Colicin E1 is a bacteriocin produced by, and lethal to, Escherichia coli that hijacks the outer membrane proteins (OMPs) TolC and BtuB to enter the cell. Colicin E1 is a bacteriocin produced by E. coli that enters the periplasm of neighboring cells and forms a pore on the cytoplasmic membrane leading to membrane depolarization and cell death. Unlike any of the other E colicins, the T domain of Colicin E1 binds to TolC, the outer membrane component of the acridine efflux pump, and the R domain binds BtuB, the primary receptor shared by all E colicins. TolC forms a large rigid conduit in the outer membrane and periplasm with a water-filled lumen.

We find that colicin E1 binds stably to TolC, not as a helical hairpin but as a single-pass folded helix with the N-terminus inside the periplasm. When resolved by cryoEM, addition of ColE1-T to TolC breaks the threefold channel symmetry and the additional protein is observed running all the way through the TolC barrel as a single-pass, all-α-helical chain spanning more than 130 Å. The ColE1 T domain inserts into TolC with its amino terminus pointing inwards through the periplasmic iris, and 2D class averages show that the carboxy terminus of the helix continues and projects out into the extracellular space. About 85 of the 190 ColE1-T residues could be modeled to this density (residues 46–131). The ColE1 chain binds TolC asymmetrically, primarily contacting only one of the three TolC chains. However, our cryoEM reconstruction of colicin E1 in complex with TolC shows that ColE1-T hinges open at the TolC box to an extended conformation upon binding to TolC (bottom). Compared to the unbound state, asymmetric ColE1 binding dilates the periplasmic TolC aperture and, makes only minor adjustments to the loops on the extracellular aperture so that they can accommodate ColE1 in the absence of any other proteins or motive force. The acidic patch of colicin E1 near the extracellular aperture contains two arginine residues (R129 and R131) that form hydrogen bond networks with one TolC chain each. In addition, colicin E1 residues T113, A116, N119, and N120 (all part of the TolC box) establish polar interactions with TolC residues G67, D69, S90, and K305 on one TolC chain (light red and light blue) while colicin H117 interacts with TolC F310 on a neighboring TolC chain (light red and light gold). By contrast with the β-barrel of TolC, in the interior of the periplasmic helical barrel of TolC, colicin E1 does not make full contact with the α-helical barrel interior and there is a gap between the two proteins.

>[3x]MKKLLPILIGLSLSGFSSLSQAENLMQVYQQARLSNPELRKSAADRDAAFEKINEARSPLLPQLGLGADYTYSNGYRDANGINSNATSASLQLTQSIFDMSKWRALTLQEKAAGIQDVTYQTDQQTLILNTATAYFNVLNAIDVLSYTQAQKEAIYRQLDQTTQRFNVGLVAITDVQNARAQYDTVLANEVTARNNLDNAVEQLRQITGNYYPELAALNVENFKTDKPQPVNALLKEAEKRNLSLLQARLSQDLAREQIRQAQDGHLPTLDLTASTGISDTSYSGSKTRGAAGTQYDDSNMGQNKVGLSFSLPIYQGGMVNSQVKQAQYNFVGASEQLESAHRSVVQTVRSSFNNINASISSINAYKQAVVSAQSSLDAMEAGYSVGTRTIVDVLDATTTLYNAKQELANARYNYLINQLNIKSALGTLNEQDLLALNNALSKPVSTNPENVAPQTPEQNAIADGYAPDSPAPVVQQTSARTTTSNGHNPFRN;> METAVAYYKDGVPYDDKGQVIITLLNGTPDGSGSGGGGGKGGSKSESSAAIHATAKWSTAQLKKTQAEQAARAKAAAEAQAKAKANRDALTQRLKDIVNEALRHNASRTPSATELAHANNAAMQAEDERLRLAKAEEKARKEAEAAEKAFQEAEQRRKEIEREKAETERQLKLAEAEEKRLAALSEEAKALEHHHHHH> TVGAV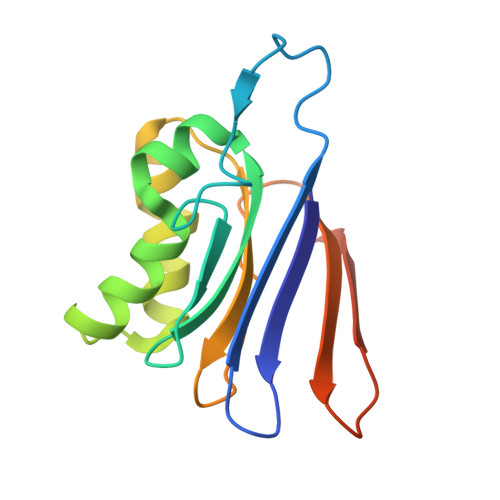ALDLDGNLAAATSTGGMTNKLPGAVGSTPLVGAGCYANNASVAVSCTGTGEVFIRALAAYDIAALMDYGGLSLAEACERVVMEKLPALGGSGGLIAIDHEGNVALPFNTEGMYRAWGYAGDTPTTGIYREKGDTVATQ1-METHYLIMIDAZOLE 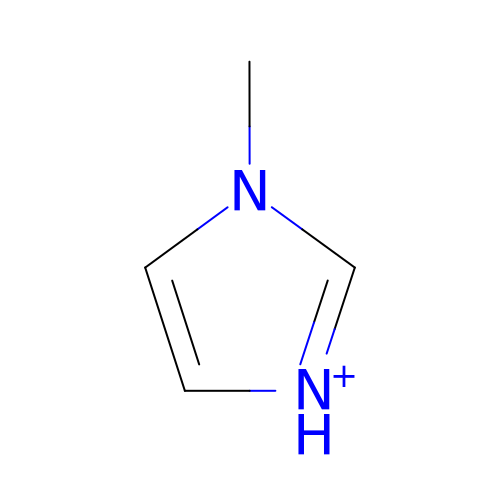| C4 H7 N2 | MCTWTZJPVLRJOU-UHFFFAOYSA-O>[4x]GPGLKQKIVIKVAMEGNNCRSKAMALVASTGGVDSVALVGDLRDKIEVVGYGIDPIKLISALRKKVGDAELLQVEQAKED;>[2x]METGNKYIEKRAIDLSRERDPNFFDNADIPVPECFWFMFKNNVRQDAGTCYSSWKMDKKVGPNWVHIKSDDNCNLSGDFPPGWIVLGKKRPGF

The rice NLR receptor Pik-1 binds the Magnaporthe oryzae effector AVR-Pik through an integrated heavy metal-associated (HMA) domain. The sensor NLR Pik-1 contains an integrated HMA domain between the CC and NB-ARC domains (Maqbool et al., 2015). Direct binding of AVR-Pik to the HMA domain is required to activate Pik-mediated immunity. However, the stealthy alleles AVR-PikC and AVR-PikF avoid interaction with Pik-HMA and evade host defenses.

The Asp67 and Lys78 polymorphisms that distinguish AVR-PikC and AVR-PikF from AVR-PikE and AVR-PikA, respectively, are located at interface 2. The crystal structure of the OsHIPP19-HMA/AVR-PikF complex revealed additional hydrogen bond interactions at interface 3 relative to integrated HMAs in the complex with AVR-Pik variants. The corresponding residue in all described Pik-1 HMA domains is serine, and while the hydroxyl group of the serine side chain only forms an intramolecular hydrogen bond within the HMA domain, the bulkier OsHIPP19Glu72 side chain extends across the interface and forms a direct hydrogen bond with the effector. By contrast, PikpSNK-EKE-HMA bound to both AVR-PikC and AVR-PikF with higher apparent affinity (larger %Rmax) than PikpNK-KE-HMA. By determining the crystal structures of the Pikp-HMASNK-EKE/AVR-PikC and Pikp-HMASNK-EKE/AVR-PikF complexes, we confirmed the formation of new contacts across the HMA/effector interface that likely account for the expanded recognition profile to AVR-PikC and AVR-PikF. Crystals were obtained in several conditions in the Morpheus screen (Molecular Dimensions), and X-ray diffraction data were collected at the Diamond Light Source (Oxford, UK) to a resolution of 2.15 Å (Pikp-HMANK-KE/AVR-PikC), 2.05 Å (Pikp-HMASNK-EKE/AVR-PikC), and 2.2 Å (Pikp-HMASNK-EKE/AVR-PikF). Interface analysis performed with qtPISA identified 15 hydrogen bonds and nine salt bridges between Pikp-HMASNK-EKE and AVR-PikC, and 16 hydrogen bonds and 11 salt bridges between Pikp-HMASNK-EKE and AVR-PikF, compared to the 12 hydrogen bonds and eight salt bridges mediating the interaction between Pikp-HMANK- KE and AVR-PikC. Inspection of the structures revealed that the side chain of Glu258 does indeed extend across the interface, forming direct hydrogen bonds with the backbone of the effectors. This single mutation also supports additional hydrogen bonds at the interface between AVR-PikC (or AVR-PikF) and residues comprising β4 of the HMA domain.>MSLNHHPIIYLVDHQKDARAALSKLLSPLD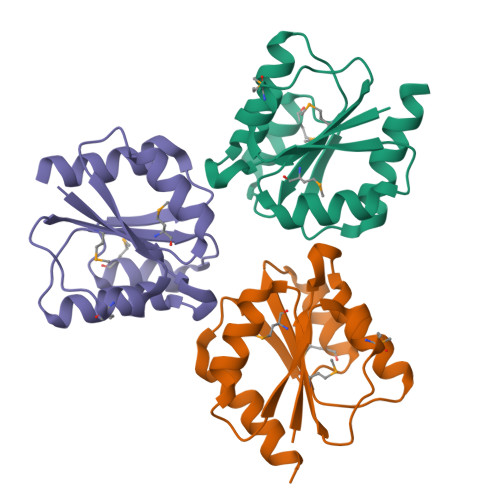VTIQCFASAESFMRQQISDDAIGMIIEAHLEDKKDSGIELLETLVKRGFHLPTIVMASSSDIPTAVRAMRASAADFIEKPFIEHVLVHDVQQIINGAKEGHHHHHH[3x]> GSPLLDDDDQVAFSFILDNIVTQKMMAVPDSWPFHHPVNKKFVPDYYKVIVNPMDLETIRKNISKHKYQSRESFLDDVNLILANSVKYNGPESQYTKTAQEIVNVCYQTLTEYDEHLTQLEKDICTAKEAALE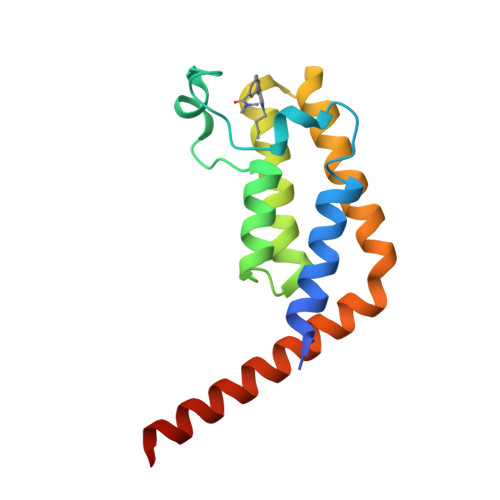EAELESLDPMT> KIGIFFSTSTGNTTEVADFIGKTLGAKA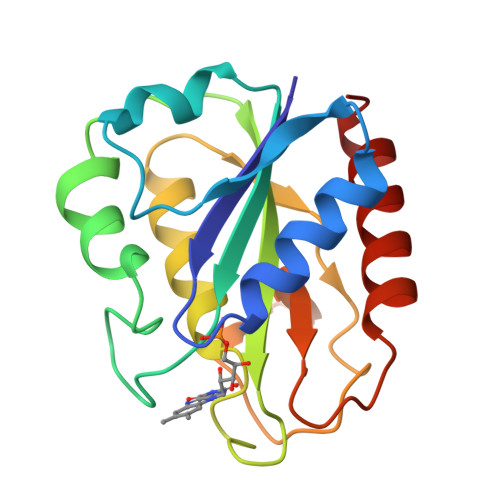DAPIDVDDVTDPQALKDYDLLFLGAPTWNTGADTERSGTSWDEFLYDKLPEVDMKDLPVAIFGLGDAEGYPDNFCDAIEEIHDCFAKQGAKPVGFSNPDDYDYEESKSVRDGKFLGLPLDMVNDQIPMEKRVAGWVEAVVSETGV> MELRHIRYFLAVAEERHFTRAAARLGIGQPPLSQQIKDLERELGALLFRRVSYGAELTEAGIAFLDVVKEIPVMAERATQAAQRAVRGELGVLRVGFTASSAFNSVVPTAIRAFRRAYPDVRLQLEEDNTTRLADGLNEGSLDVAFLRPGFAGSERFHLRMLSEEPMMIVMAENHPAASYEEISLSAFRDETFLLFPR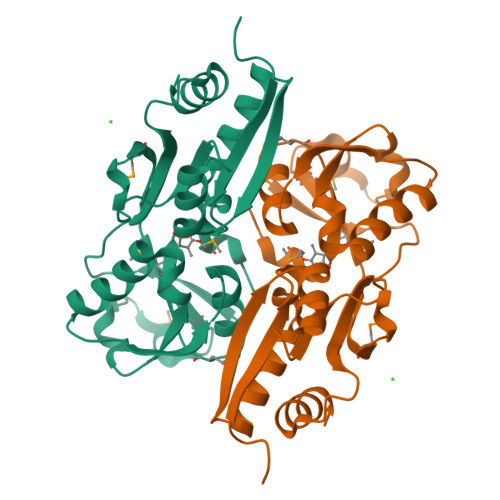EIGLTLYDSVIESCRTAGFEPTIGQLAPQIASVINLVAAEMGVSIVPASMSQVKVIGVVYRHIADQTPTAKLALAYRRGDTSPVLRNFVLTVFP>TGGRNSIRYSELAPLFDTTRVYLVDNKSTDVASLNYQNDHSNFLTTVIQNNDYSPGEASTQTINLDDRSHWGGDLKTILHTNMPNVNEFMFTNKFKARVMVSRSLTKDKQVELKYEWVEFTLPEGNYSETMTIDLMNNAIVEHYLKVGRQNGVLESDIGVKFDTRNFRLGFDPVTGLVMPGVYTNEAFHPDIILLPGCGVDFTHSRLSNLLGIRKRQPFQEGFRITYDDLEGGNIPALLDVDAYQASLKDDTEQGGDGAGGGNNSGSGAEENSNAAAAAMQPVEDMNDHAIRGDTFATRAEEKRAEAEAAAEAAAPAAQPEVEKPQKKPVIKPLTEDSKKRSYNLISNDSTFTQYRSWYLAYNYGDPQTGIRSWTLLCTPDVTCGSEQVYWSLPDMMQDPVTFRSTSQISNFPVVGAELLPVHSKSFYNDQAVYSQLIRQFTSLTHVFNRFPENQILARPPAPTITTVSENVPALTDHGTLPLRNSIGGVQRVTITDARRRTCPYVYKALGIVSPRVLSSRTF[5x];>[12x]ATPSMMPQWSYMHISGQDASEYLSPGLVQFARATETYFSLNNKFRNPTVAPTHDVTTDRSQRLTLRFIPVDREDTAYSYKARFTLAVGDNRVLDMASTYFDIRGVLDRGPTFKPYSGTAYNALAPKGAPNPCEWDEAATALEINLEEEDDDNEDEVDEQAEQQKTHVFGQAPYSGINITKEGIQIGVEGQTPKYADKTFQPEPQIGESQWYETEINHAAGRVLKKTTPMKPCYGSYAKPTNENGGQGILVKQQNGKLESQVEMQFFSTTEATAGNGDNLTPKVVLYSEDVDIETPDTHISYMPTIKEGNSRELMGQQSMPNRPNYIAFRDNFIGLMYYNSTGNMGVLAGQASQLNAVVDLQDRNTELSYQLLLDSIGDRTRYFSMWNQAVDSYDPDVRIIENHGTEDELPNYCFPLGGVINTETLTKVKPKTGQENGWEKDATEFSDKNEIRVGNNFAMEINLNANLWRNFLYSNIALYLPDKLKYSPSNVKISDNPNTYDYMNKRVVAPGLVDCYINLGARWSLDYMDNVNPFNHHRNAGLRYRSMLLGNGRYVPFHIQVPQKFFAIKNLLLLPGSYTYEWNFRKDVNMVLQSSLGNDLRVDGASIKFDSICLYATFFPMAHNTASTLEAMLRNDTNDQSFNDYLSAANMLYPIPANATNV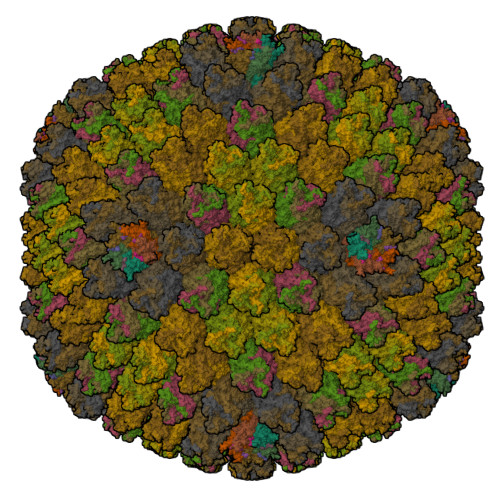PISIPSRNWAAFRGWAFTRLKTKETPSLGSGYDPYYTYSGSIPYLDGTFYLNHTFKKVAITFDSSVSWPGNDRLLTPNEFEIKRSVDGEGYNVAQCNMTKDWFLVQMLANYNIGYQGFYIPESYKDRMYSFFRNFQPMSRQVVDDTKYKDYQQVGILHQHNNSGFVGYLAPTMREGQAYPANFPYPLIGKTAVDSITQKKFLCDRTLWRIPFSSNFMSMGALTDLGQNLLYANSAHALDMTFEVDPMDEPTLLYVLFEVFDVVRVHRPHRGVIETVYLRTPFSAGNATT;>[5x]TFNPVYPYDT CDT is a member of the Iota family of protein toxins which also consists of two homologous toxins produced by Clostridium perfringens (the Iota toxin) and Clostridium spiroforme (C. spiroforme Transferase, CST). All three Iota toxin family members are assembled from two polypeptide chains termed the “A” subunit (CDTa, Ia, and CSTa) and “B”, subunit (CDTb, Ib, and CSTb). All three B subunits are presumed to contain five domains that are involved in regulation (D1), oligomerization (D2 and D3), and host recognition (D3’ and D4). Once proteolyzed, the mature form of CDTb forms a large heptameric, soluble structure referred to as the prepore which binds one molecule of CDTa to generate the toxic moiety, CDT.

A map of the CDTb trimer was refined to a final resolution of 4.19 Å. Although the nominal resolution of the final map is lower than the initial reconstruction, the final map does not suffer from problems arising from preferred orientation as is apparent in the initial map. The model of the dimer was used as a reference to generate a molecular model of the trimeric intermediate. We note a similar arrangement of Chains A and B within this structure and the presence of a third chain, ‘Chain C’, positioned next to Chain B, opposite of Chain A. As observed in the dimeric structure, the orientations of all three chains are rotated compared to the assembled, symmetric heptamer with an observed rotation of ~40° about the central pseudosymmetry axis between Chains A and B and ~43° between Chains B and C. The interface between Chains A and B and Chains B and C mirror those of the dimeric intermediate and do not indicate the presence of additional recognition elements. Interestingly, a helical pitch is also observed within the trimer wherein Chain C is positioned ~4 Å out of plane when compared to the symmetric structure.

>[3x]MKIQMRNKKVLSFLTLTAIVSQALVYPVYAQTSTSNHSNKKKEIVNEDILPNNGLMGYYFTDEHFKDLKLMAPIKDGNLKFEEKKVDKLLDKDKSDVKSIRWTGRIIPSKDGEYTLSTDRDDVLMQVNTESTISNTLKVNMKKGKEYKVRIELQDKNLGSIDNLSSPNLYWELDGMKKIIPEENLFLRDYSNIEKDDPFIPNNNFFDPKLMSDWEDEDLDTDNDNIPDSYERNGYTIKDLIAVKWEDSFAEQGYKKYVSNYLESNTAGDPYTDYEKASGSFDKAIKTEARDPLVAAYPIVGVGMEKLIISTNEHASTDQGKTVSRATTNSKTESNTAGVSVNVGYQNGFTANVTTNYSHTTDNSTAVQDSNGESWNTGLSINKGESAYINANVRYYNTGTAPMYKVTPTTNLVLDGDTLSTIKAQENQIGNNLSPGDTYPKKGLSPLALNTMDQFSSRLIPINYDQLKKLDAGKQIKLETTQVSGNFGTKNSSGQIVTEGNSWSDYISQIDSISASIILDTENESYERRVTAKNLQDPEDKTPELTIGEAIEKAFGATKKDGLLYFNDIPIDESCVELIFDDNTANKIKDSLKTLSDKKIYNVKLERGMNILIKTPTYFTNFDDYNNYPSTWSNVNTTNQDGLQGSANKLNGETKIKIPMSELKPYKRYVFSGYSKDPLTSNSIIVKIKAKEEKTDYLVPEQGYTKFSYEFETTEKDSSNIEITLIGSGTTYLDNLSITELNSTPEILDEPEVKIPTDQEIMDAHKIYFADLNFNPSTGNTYINGMYFAPTQTNKEALDYIQKYRVEATLQYSGFKDIGTKDKEMRNYLGDPNQPKTNYVNLRSYFTGGENIMTYKKLRIYAITPDDRELLVLSVD2-(3-{[4-(HYDROXYAMINO)-2-METHYLPYRIMIDIN-5-YL]METHYL}-4-METHYL-2,3-DIHYDRO-1,3-THIAZOL-5-YL)ETHYL TRIHYDROGEN DIPHOSPHATE | C12 H19 N4 O8 P2 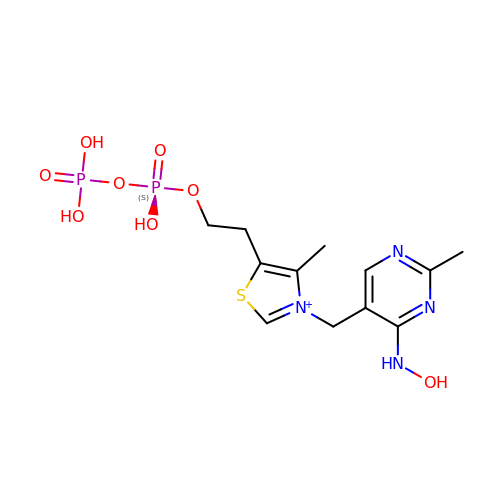S | YVLOFEOVSMJZTD-UHFFFAOYSA-O>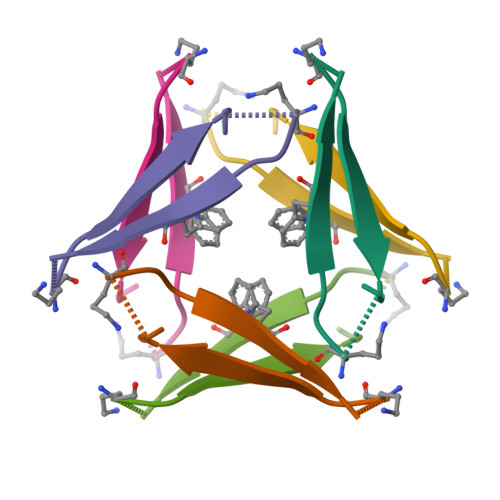 VAKLVFFADAAIIGLM> SMANLDTQFQEFYGELQITVTKKQALITSHNNLRTKIQKYFAKNHPEYVPSFYIQGSYKMGTTIRTRDDECDLDDGCYFIPKPEVKGITLQNWVMDAVNGTVGATPVHKNKCIRVNYAAGYHIDLPVYRKERCNDNTEHPELAVRDGEYELSDPREIVQWFNSKKKDNPVLIRLVSYLKSWCDTVRGFMPPGLAMTILASKYQKKHEGRDDIALRDTLKS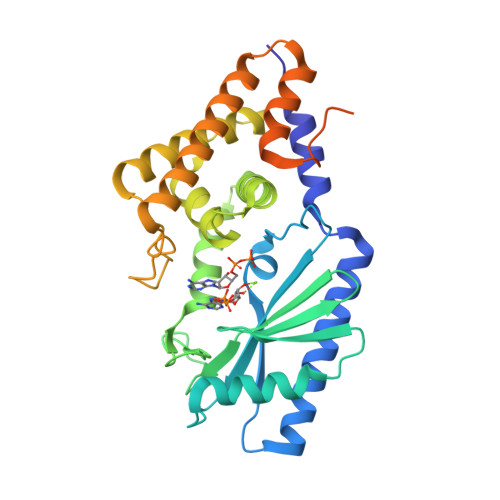IRTALQANFSCVVPGTPYDDLFESYDSNRQEKFMSELNGFIEDADRAVNEKNKLKASKLWKKHLGNRFHLAPDENDAEMSKLDKLRDIGNKVLTGIATTAHNGYIHAAEGVKNVSHRNYGN>GMYLEKLQQWRYATADFSGAHITDDVLDKLLNTTRLTASSYGLQPYCTLVIRNKGLREQLVNHSFGQQKVADSSALVIFAAKTGAVADIVDPYISELSQQRQLTNEEAENTRNYFTQKLQAMSAATRKEWAVRQAYIGLGTFLLAAAELEVDSCPMEGIEHDAYDNILSLKDLGLSTVFACPVGYRSEADTTQF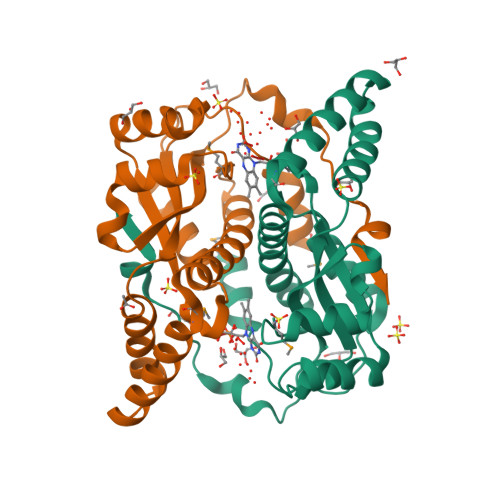QKKVRQPLSRFKVVL[3x]> APPGLVGALPPVGFFDPAGFAAKASPEELSRYREVEIMHGRFAQLAVLGFIIPEKCAYDGSFGDDFLAPTGRALEVFNTDPLWLGLTLAVISALETVRLIETEPGTRTDAKIESLGWRPKTESEYINYQVRELQQGRLAMLAFAGEVAQELVNDKPLLVNLQDSGFVSW;> FENELGVIAPTGFFDPLGFTQDIDQEKFDQYRTAELKHGRVAQLAVVGYVVPEFFRWGFDIAPGIACADVPNGVAAINAIPALGWAQIIFAIGAVDVRGWFGNFDIGKPDLKGKEEERALQELQHGRLAMLAILELLRHDSQNLVKPGFDGLDNLITGLPFLYN;> FENELGVIAPTGFFDPLGLSKNISKEKFDEYRTAELKHGRAAMLAVLGYIAPETYRFGFDIAPGVSTYDIPNGVAAIDYIPALGWAQIIFLIGAVDYWGVLGDFSFGKPDLGDKEEERKLQELQHGRLAMLAFLELLRHDSQNFVSPGFDGYDKMITGLPFMYG

Diatoms are dominant marine algae and contribute around a quarter of global primary productivity, the success of which is largely attributed to their photosynthetic capacity aided by specific fucoxanthin chlorophyll-binding proteins (FCPs) to enhance the blue-green light absorption under water. One of the important factors responsible for the powerful vitality of diatoms is their extraordinary light-harvesting capacity, which is achieved by their unique antenna system, fucoxanthin (Fx) chlorophyll (Chl) c binding proteins (FCPs). Here, we solved the structures of a PSII-FCPII supercomplex and a trimeric FCP from C. meneghiniana by single particle analysis using cryo-EM, which revealed detailed structures of monomeric, dimeric and trimeric FCPs, as well as their binding to the PSII core. In conclusion, the cryo-EM structures of PSII-FCPII and the trimeric FCP of C. meneghiniana provide detailed insights into the structures of various FCP antennae and the assembly of FCPs within the PSII supercomplex.

Based on the analysis of the FCP bands by mass spectrometry and specific sequences obtained via transcriptome sequencing of C. meneghiniana and genomic sequence of C. cryptica, we assigned three FCP sequences to the local map of FCPII-G/H1/H2 adjacent to CP47/D2/PsbX/PsbH as Cc-Lhcx6_1, Cm-Lhcf7 and Cc-Lhcf7-like protein, respectively. The B-C loop of FCPII-G is short and shifted towards its helix-A on the lumenal surface, leaving a large space to accommodate PsbX. Helix C of FCPII-G interacts closely with PsbX by a strong hydrogen bond and extensive hydrophobic interactions. We assigned 11 Chls a and 3 carotenoid sites in Cm-FCPII-G. One Dtx is identified at the 303 site of FCPII-G in the current structure, which shares the same location and orientation as Ddx303 in Cg-FCPII-D. Cm-FCPII-H1/H2 was identified as a heterodimer, despite of 80% sequence identity between them. FCPII-H1/H2 dimer is assembled in a “head-to-head” manner by two adjacent helices C, which resembles the Pt-Lhcf4 dimer. The binding of the FCPII-H dimer to the PSII core is dominated by the association of FCPII-H1 with FCPII-G in their loop regions with help of several crucial residues and pigments. Four carotenoids are assigned in each of FCPII-H1 and FCPII-H2, they are Fx 301/302 and Ddx 303/305. Thus FCPII-G and FCPII-H are both inner FCP antennae strongly associated with the PSII core and probably mediate EET from outside FCPs, and may also play photoprotection roles through the Ddx-Dtx cycle under high light conditions.>SVSYDGERRVNFNENWRFQRETNGSIAGAQNPGFDDSSWRKLNLPHDWSIELDFNKNSLATHEGGYLDGGIGWYRKTFTIPESMKGKRISLDFDGVYMNSTTYLNGEVLGTYPFGYNAFSYDISDKLYKDGRANVLVVKVNNTQPSSRWYSGSGIYRNVYLTVTDPIHVARYGTFVTTPNLEKSIKEDRADVNIKTKISNDAAEAKQVKIKSTIYDGAGNTVQTVETEEKTAAAGTVTPFEQNTVIKQPKLWSIDKPYRYNLVTEVIVGGQTVDTYETKFGVRYFKFDENEGFSLNGEYMKLHGVSMHHDLGALGAATNARGVERQMQIMKDMGVNAIRVTHNPASPELLEAANKLGLFIIEEAFDSWAQSKKPYDYGRFFNAWAEHDIKEMVDRGKNEPAIIMWSIGNEIYDTTNAAGVETARNLVGWVKEIDTTRPTTIGEDKTRGDKVNVTPINSYIKEIFNIVDVVGLNYSENNYDGYHKQNPSWKLYGSETSSATRSRGVYTHPYQYNQSTKYADLQQSSYDNDYVGWGRTAEDAWKYDRDLKHIAGQFIWTGFDYIGEPTPYYNSYPAKSSYFGAVDTAGFPKDIFYYYQSQWKKEPMVHLLPHWNWKEGEKVRVLAYTNASKV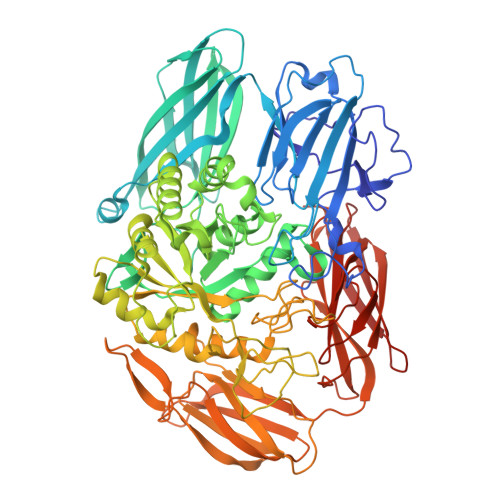ELVLNGESLGEKNYDNKQTSWGAPYKETKDGKTYLEWAVPFKPGKLEAVAKDENGKVIARDQVVTAGEPASVRLTADRKVVKADGTDLSFITADIVDSKGIVVPDADHLITFNVTGQGELAGVDNGNASSVERYKDNKRKAFSGKALAIVQSSKLSGKITVHASVAGLSSDSTSVFTVTP[2x]>[2x]SLDKLHVTSTRPQYVRIKNWGSGEILHDTLHHKATSDFTCKSKSCLGSIMNPKSLTRGPRDKPTPLEELLPHAIEFINQYYGSFKEAKIEEHLARLEAVTKEIETTGTYQLTLDELIFATKMAWRNAPRCIGRIQWSNLQVFDARNCSTAQEMFQHICRHILYATNNGNIRSAITVFPQRSDGKHDFRLWNSQLIRYAGYQMPDGTIRGDAATLEFT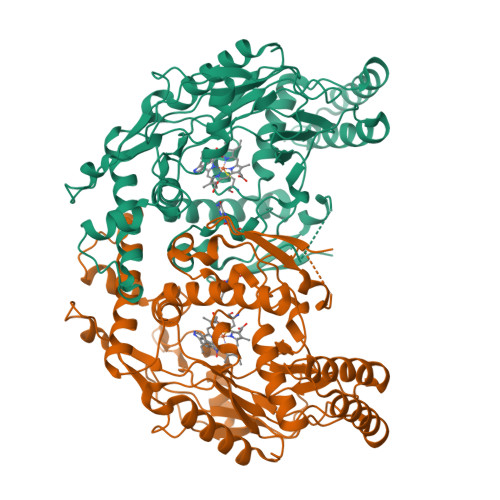QLCIDLGWKPRYGRFDVLPLVLQADGQDPEVFEIPPDLVLEVTMEHPKYEWFQELGLKWYALPAVANMLLEVGGLEFPACPFNGWYMGTEIGVRDFCDTQRYNILEEVGRRMGLETHTLASLWKDRAVTEINVAVLHSFQKQNVTIMDHHTASESFMKHMQNEYRARGGCPADWIWLVPPVSGSITPVFHQEMLNYVLSPFYYYQIEPWKTHIWQNE> EVNKIIGSRTAGEGAMEYLIEWKDGHSPSWVPSSYIAADVVSEYETPWWTAARKADEQALSQLLEDRDVDAVDENGRTALLFVAGLGSDKCVRLLAEAGADLDHRDMRGGLTALHMAA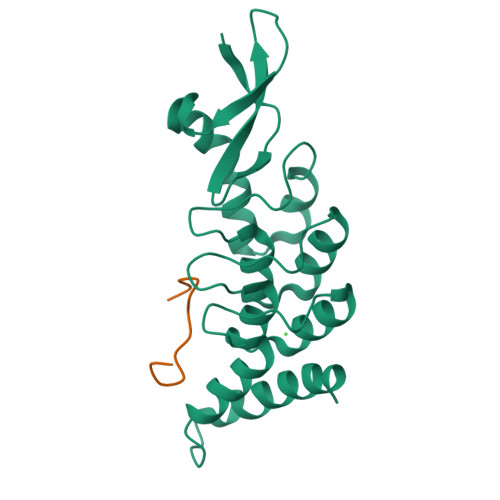GYVRPEVVEALVELGADIEVEDERGLTALELAREILKTTPKGNPMQFGRRIGLEKVINVLEGQVF;> YPGGSFDPLGLA>LSDSRVLWAPAEAHPLSPQGHPARLHRIVPRLRDVFGWGNLTCPICKGLFTAINLGLKKEPNVARVGSVAIKLCNLLKIAPPAVCQSIVHLFEDDMVEVWRRSVLSPSEACGLLLGSTCGHWDIFSSWNISLPTVPKPPPKPPSPPAPGAPVSRILFLTDLHWDHDYLEGTDPDCADPLCCRRGSGLPPASRPGAGYWGEYSKCDLPLRTLESLLSGLGPAGPFDMVYWTGDIPAHDVWHQTRQDQLRALTTVTALVRKFLGPVPVYPAVGNHESTPVNSFPPPFIEGNHSSRWLYEAMAKAWEPWLPAEALRTLRIGGFYALSPYPGLRLISLNMNFCSRENFWLLINSTDPAGQLQWLVGELQAAEDRGDKVHIIGHIPPGHCLKSWSWNYYRIVARYENTLAAQFFGHTHVDEFEVFYDEETLSRPLAVAFLAPSATTYIGLNPGYRVYQIDGNYSGSSHVVLDHETYILNLTQANIPGAIPHWQLLYRARETYGLPNTLPTAWHNLVYRMRGDMQLFQTFWFLYHKGHPPSEPCGTPCRLATL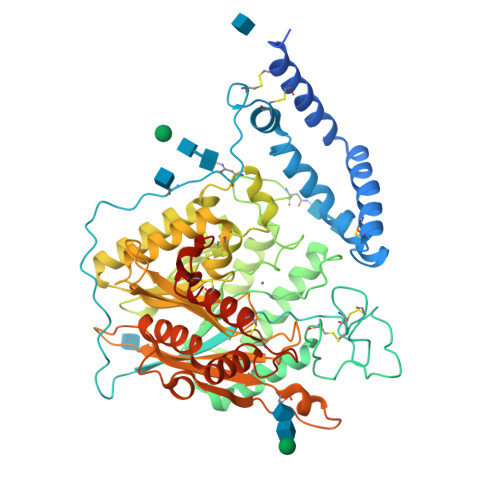CAQLSARADSPALCRHLMPDGSLPEAQSLWPRPLFC[3x]>[3x]GSHMPGFYEIVIKVPSDLDEHLPGISDSFVNWVAEKEWELPPDSDMDLNLIEQAPLTVAEKLQRDFL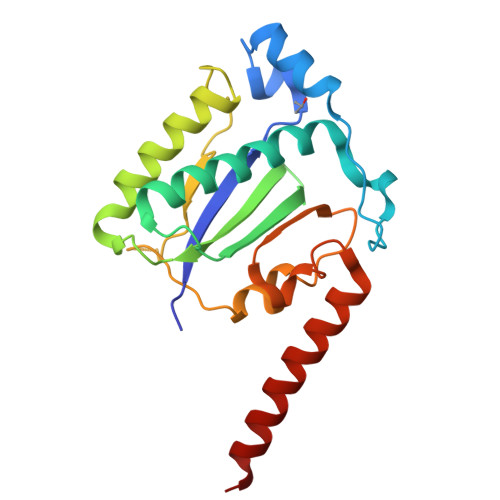TEWRRVSKAPEALFFVQFEKGESYFHMHVLVETTGVKSMVLGRFLSQIREKLIQRIYRGIEPTLPNWFAVTKTRNGAGGGNKVVDESYIPNYLLPKTQPELQWAWTNMEQYLSACLNLTERKRLVAQHLTHVSQTQEQNKEN> ALPAKENEGCIVSVNSGKRYCLPVGQRSGYSLPDWIVGQEVYVDSGAKAKVLLSDWDNLSYNRIGEFVGNV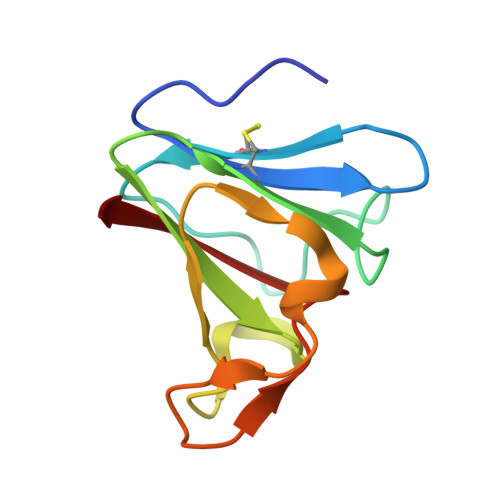NPADMKKVKAWNGQYLDFSKPRSMRVVYK> SRTGYDNREIVMKYIHYKLSQ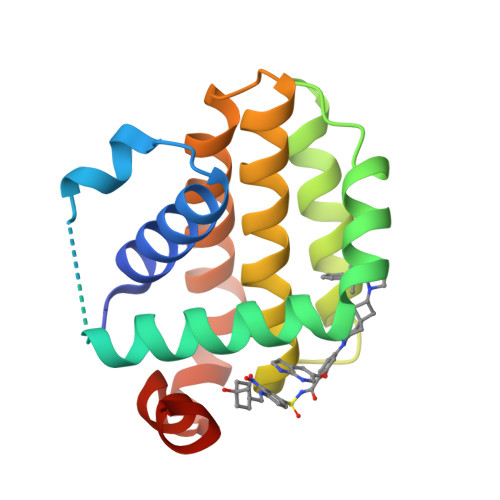RGYEWDAGDDVEENRTEAPEGTESEVVHLTLRQAGDDFSRRYRRDFAEMSSQLHLTPFTARGRFATVVEELFRDGVNWGRIVAFFEFGGVMCVESVNREMSPLVDNIALWMTEYLNRHLHTWIQDNGGWDAFVELYGPSMR> EDASRMEE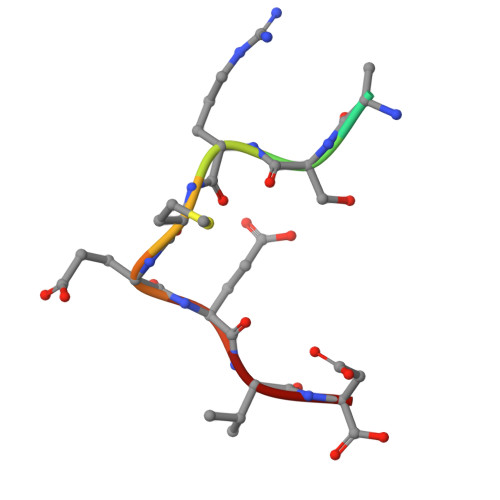VD> MAHAGRTGYDNREIVMKYIHYKLSQRGYEWDAGDDVEENR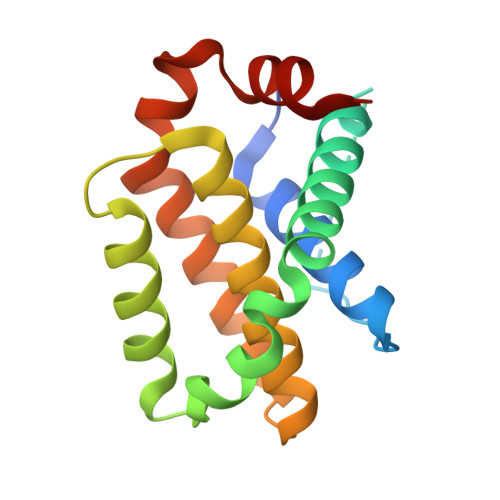TEAPEGTESEVVHLTLRQAGDDFSRRYRRDFAEMSSQLHLTPFTARGRFATVVEELFRDGVNWGRIVAFFEFGGVMCVESVNREMSPLVDNIAIWMTEYLNRHLHTWIQDNGGWDAFVELYGPSMR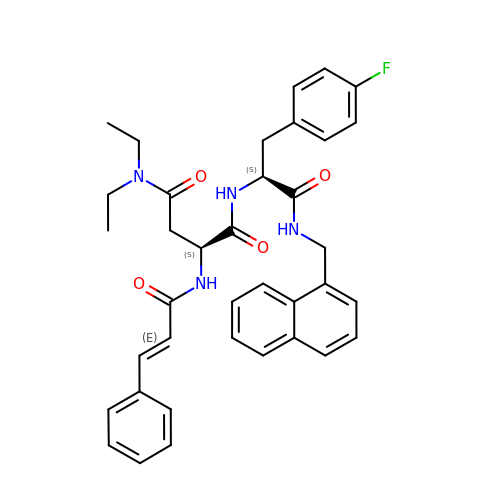N,N-diethyl-N~2~-[(2E)-3-phenylprop-2-enoyl]-L-asparaginyl-4-fluoro-N-[(naphthalen-1-yl)methyl]-L-phenylalaninamide | C37 H39 F N4 O4 | GDEDTAMXMSKSNF-DBGGJHLHSA-N> MKELMRNVYLLDDTLVTKSKYGSHYGEKVFDGYREWVPWRSKLAAMILKGHRLKLRGDERVLYLGAASGTTVSHLADIVDEGIIYAVEYSAKPFEKLLELVRERNNIIPLLFDASKPWKYSGIVEKVDLIYQDIAQKNQIEILKANAEFFLKEKGEV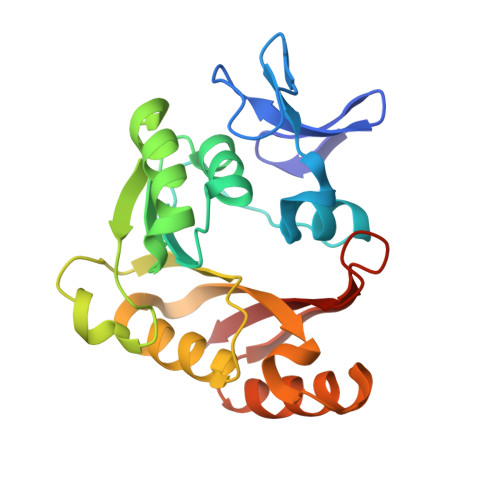VIMVKARSIDSTAEPEEVFKSVLKEMEGDFKIVKHGSLMPYHRDHIFIHAYRF>KHSLPDLPYDYGALEPHINAQIMQLHHSKHHAAAVNNLNVTEEKYQEALAKGDVTAQIALQPALKFNGGGHINHSIFWTNLSPNGGGEPKGEL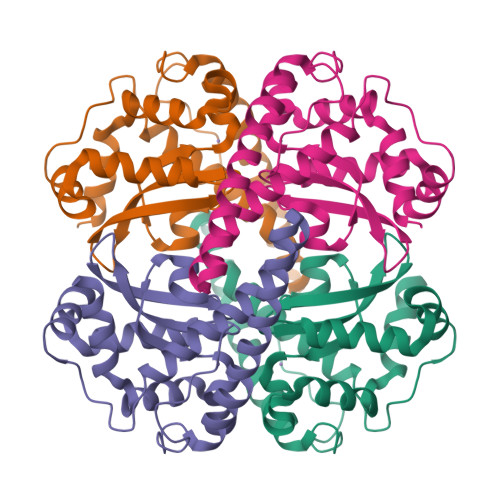LEAIKRDFGSFDKFKEKLTAASVGVQGSGWGWLGFNKERGHLQIAACPNQDPLQGTTGLIPLLGIDVWEHAYYLQYKNVRPDYLKAIWNVINWENVTERYMACKK[2x]>FADDHAMSPDMKLLAGASNWVNQSGSVAQFVFTPSPTQPQTYEVSGNYINNAQGTGCKGTPYPLSGAYYSGNQIISFSVVWSNASANCQSATGWTGYFDFSGSQA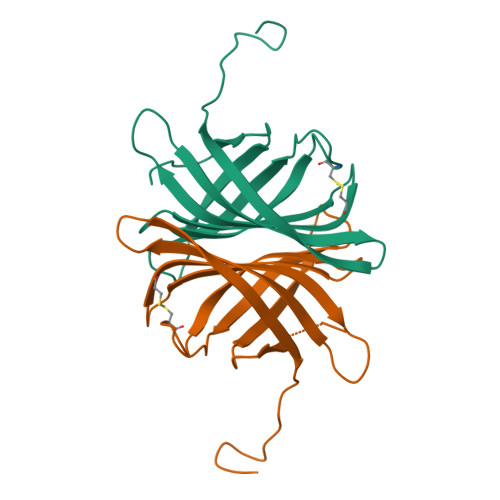VLKTDWNLAFYSGSTPAIQQGQDDFMQSVATVSESLLTE[2x]> GSGAMAQNLDSMLHGTGMKSDSDQKKSENGVTLAPEDTLPFLKCYCSGHCPDDAINNTCITNGHCFAIIEEDDQGETTLTSGCLGLEGSDFQCRDTPIPHQRRSIECCRTNLCNQYL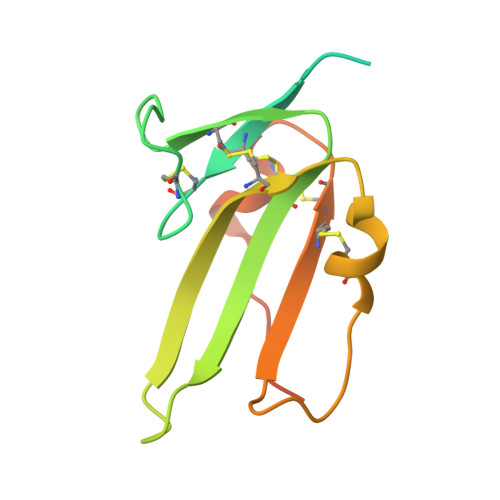QPTLPPVVIGPFFDGSIR>MTLQEQIMKALHVQPVIDPKAEIRKRVDFLKDYVKKTGAKGFVLGISGGQDSTLAGRLAQLAVEEIRNEGGNATFIAVRLPYKVQKDEDDAQLALQFIQADQSVAFDIASTVDAFSNQYENLLDESLTDFNKGNVKARIRMVTQYAIGGQKGLLVIGTDHAAEAVTGFFTKFGDGGADLLPLTGLTKRQGRA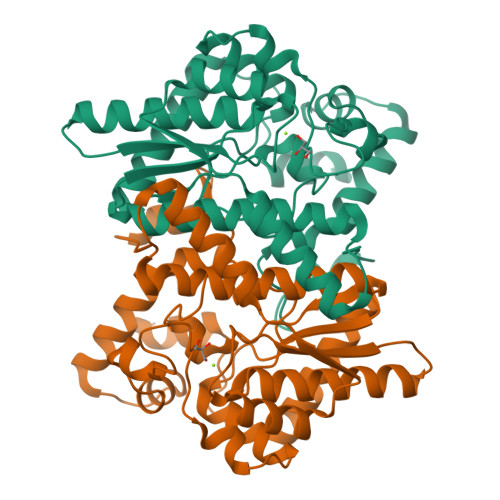LLQELGADERLYLKMPTADLLDEKPGQADETELGITYDQLDDYLEGKTVPADVAEKIEKRYTVSEHKRQVPASMFDDWWKLAAALEHHHHHH[2x]>[4x]PDARSDARDLTAFQKNILTVLGEEA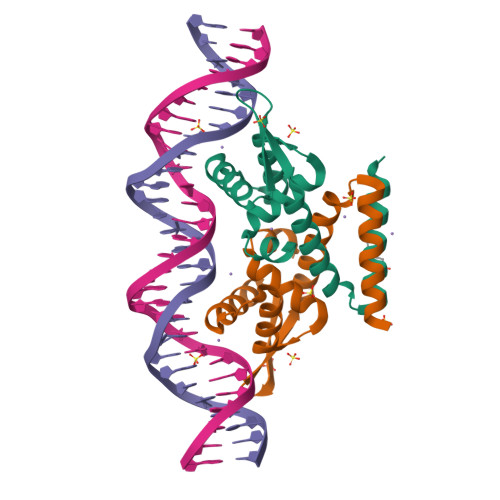RYGLAIKRELEEYYGEEVNHGRLYPNLDDLVNKGLVEKSELDKRTNEYALTNEGFDAVVDDLEWTLSKFVADADRRERVETIVADDAAALE The bacterial CYP105 family is involved in secondary metabolite biosynthetic pathways and plays essential roles in the biotransformation of xenobiotics. This study investigates the newly identified H2O2-mediated CYP105D18 from Streptomyces laurentii as the first bacterial CYP for N-oxidation. The CYP105 family is involved in biosynthetic pathways of secondary metabolites and biotransformation of xenobiotic compounds.

Crystallization experiments for full-length CYP105D18 yielded crystals in the space group C2 diffracting to 1.7 Å. A Ramachandran plot analysis of the refined model showed that 96.55 and 0% of non-glycine residues were in favored regions and outliers, respectively. The final model of CYP105D18 exhibited electron density for most of the molecule, except for the N-terminus (amino acids 1–3) and a loop containing residues 73–85, which connected αB and αC [dotted line in Fig. 5(a)]. The asymmetric unit had one molecule of CYP105D18. A flexible, less structured loop was observed in the B/C loop, and electron density for residues 73–84 was absent from the substrate-free structure, indicating that this region had a high degree of flexibility. Taken to­gether, these findings show that the B/C loop in the active site of the CYP105D18 structure was flexible and remained in an open confirmation without substrate. Across from the heme molecule are Phe338 and Gln348, which correspond to Phe441 and Gln451 of P450 4B1 and show a closed conformation. Notably, the substrate-free CYP105D18 shows a small blob on the heme molecules, as depicted in Fig. 6, indicating that the heme of CYP105D18 is oxidized. Structural comparisons between the substrate-free and complex forms of CYP105D18s revealed that conformation changes occurred mainly in the B/C loop region.

> MTEAVAFPQNRSCPYHPPTAYEPLREERPLSRVTLWNGRQVWFVTGHQAARALLGDQRLSTDSTREDFPLPTERSESLRRQRRGALLGWDDPEHNEQRRMLIPSFTLRRAESMRPRIQAIVDRLLDDMIAAGPSAELVGAFALPVPSMVICELLGVPYGDHEFFEEQSRRLLRGPAAEDIEKAFRSLEGYFGELIETKRTDPGEGVIDDLVARQREEGRPDDDELVQFATVLLVAGHETTANMISLATYTLLEHPARLAELRADPGLVPAAVEELLRFLSIADGLVRVAREDVPVGDQVIRAGEGVVFPTSLINRDDSVYEHPDTLDWSRSARHHVAFGFGIHQCLGQNLARIELEIALGTLLRRLPGLRLAAPADRIPFKPGDTIQGMLELPVTW(4R)-4-[(3R,5R,8R,9S,10S,13R,14S,17R)-10,13-dimethyl-3-(2-methyl-2-oxidanyl-propyl)-2,3,4,5,6,7,8,9,11,12,14,15,16,17-tetradecahydro-1H-cyclopenta[a]phenanthren-17-yl]pentanoic acid | 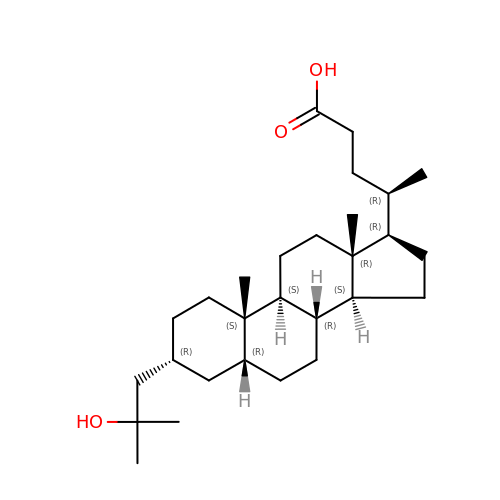C28 H48 O3 | YEJWIEPCSOSHIJ-CUYCEIPOSA-N[(3~{S})-2,2-dimethyl-3-oxidanyl-4-oxidanylidene-4-[[3-oxidanylidene-3-[2-(prop-2-enoylamino)ethylamino]propyl]amino]butyl] dihydrogen phosphate | C14 H26 N3 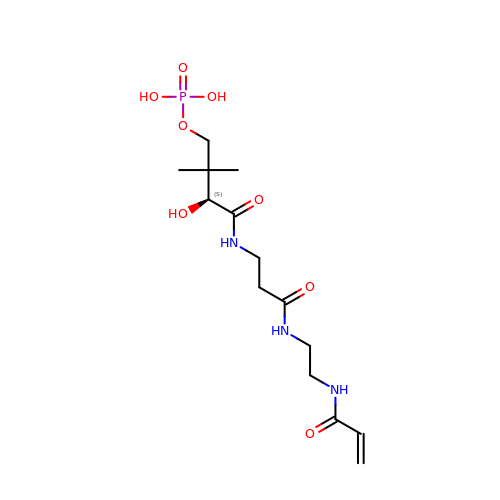O8 P | BHBIKTJIKWGGMD-GFCCVEGCSA-N> 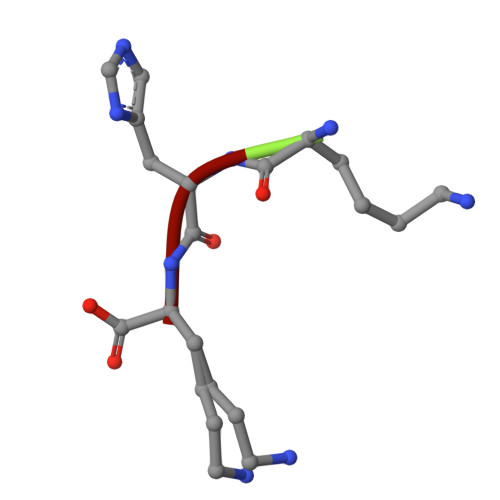KHK>GSMEKAAVNEDGLVIPLIDFSKFLEGDETLKLETAKAILHGFQTAGFIYLKNIPIQPDFREHVFNTSAKFFKLPKEKKLEVGWTTPEANRGYSAPGREKVTQLTDPAEIEKIRSAAPDIKESYEIGREDEPGHPNPWPAEQDDLVGFKSTMNNFFDQCKALHIEVMRAIAVGMGIDANYFDSFVDVGDNILRLLHYPAVKSEVFKINPGQVRAGEHTDYGSITLLFQDSRGGLQVKSPNGQFIDATPIENTVVVNAGDLLARWSNDTIKSTVHRVVEPPKQEDVHPPRYSIAYFCNPNHKSYIEAIPGTYAAESERKYEGINSGKYLVQRLAATYLEHHHHHH[4x]

Like the TET proteins, T7H is also a Fe2+ and α-KG dependent dioxygenase. Here we report the crystal structures of N. crassa T7H (NcT7H) in apo form, in α-KG-bound form and in complexes with α-KG and T, 5hmU or 5fU. Similar to other α-KG dependent dioxygenases, NcT7H adopts a variation of double-stranded β-helix (DSBH) fold as the core. The active site of NcT7H is located at the front end (opposite to the back end) of the DSBH core and partially covered by the α10 helix at the C-terminus.

The crystal structures of the full-length NcT7H in complex with α-KG (NcT7H-AKG), and in complexes with α-KG and T (NcT7H-T), with α-KG and 5hmU (NcT7H-5hmU), and with α-KG and 5fU (NcT7H-5fU) were solved by the MR method at 2.1 Å, 2.05 Å, 2.35 Å, and 2.15 Å resolution, respectively. In all these structures, the asymmetric unit contains four NcT7H molecules, of which two molecules consist of the whole polypeptide chain and the other two have a disordered region (approximately residues 94–114) due to differed crystal packing environments. In addition, similar to the apo NcT7HΔC structure, a metal ion is bound at the active site, which is assigned as Ni2+ owing to the presence of NiCl2 in the crystallization solution and the verification of the ICP-AES analysis. Structural comparison shows that the α-KG binding does not cause significant conformational changes in the overall structure (RMSD of <1.0 Å for all Cα atoms) but induces small conformational changes at the active site. Compared to the apo NcT7HΔC structure, in the α-KG-bound NcT7H structure, the residues composing the active site and the associated β-strands move slightly towards α-KG, and the active site assumes a relatively more compact conformation. In the ligand-bound NcT7H structures, the Ni2+ retains the coordinations with the three residues and one water molecule (Wat1), but the other two water molecules are replaced by the C1-carboxylate and C2-oxo groups of α-KG. In the ligand-bound NcT7H structures, α-KG binds to a positively charged pocket with the C5-carboxylate embedded in the pocket and the C1-carboxylate oriented towards the substrate. The C5-carboxylate is stabilized by four hydrogen-bonding interactions with the side chains of Tyr194, Arg286 and Ser288. The C1-carboxylate forms a hydrogen bond with the side chain of Arg190. In the α-KG-bound NcT7H structure, the C3 atom of α-KG is about 3.6 Å away from the hydroxyl group of Tyr194.>[2x]ERRRGLTDPEMAAVILKALPEAPLDGNNKMGYFVTPRWKRLTEYEALTVYAQPNADWIAGGLDWGDWTQKFHGGRPSWGNETTELRTVDWFKHRDPLRRWHAPYVKDKAEEWRYTDRFLQGYSADGQIRAMNPTWRDEFINRYWGAFLFNEYGLFNAHSQGAREALSDVTRVSLAFWGFDKIDIAQMIQLERGFLAKIVPGFDESTAVPKAEWTNGEVYKSARLAVEGLWQEVFDWNESAFSVHAVYDALFGQFVRREFFQRLAPRFGDNLTPFFINQAQTYFQIAKQGVQDLYYNCLGDDPEFSDYNRTVMRNWTGKWLEPTIAALRDFMGLFAKLPAGTTDKEEITASLYRVVDDWIEDYASRIDFKADRDQIVKAVLAGLK;>[2x]AANRAPTSVNAQEVHRWLQSFNWDFKNNRTKYATKYKMANETKEQFKLIAKEYARMEAVKDERQFGSLQVALTRLNAGVRVHPKWNETMKVVSNFLEVGEYNAIAATGMLWDSAQAAEQKNGYLAQVLDEIRHTHQCAYVNYYFAKNGQDPAGHNDARRTRTIGPLWKGMKRVFSDGFISGDAVECSLNLQLVGEACFTNPLIVAVTEWAAANGDEITPTVFLSIETDELRHMANGYQTVVSIAN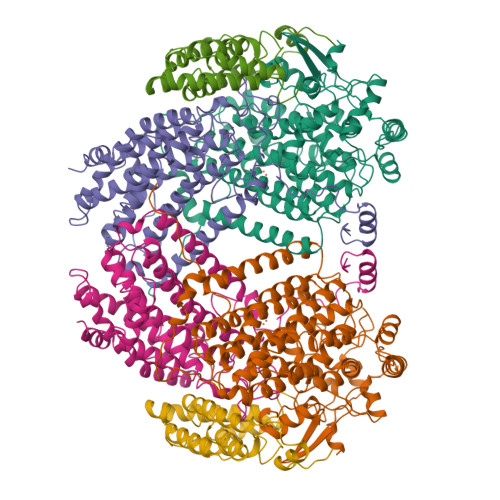DPASAKYLNTDLNNAFWTQQKYFTPVLGMLFEYGSKFKVEPWVKTWDRWVYEDWGGIWIGRLGKYGVESPRSLKDAKQDAYWAHHDLYLLAYALWPTGFFRLALPDQEEMEWFEANYPGWYDHYGKIYEEWRARGCEDPSSGFIPLMWFIENNHPIYIDRVSQVPFCPSLAKGASTLRVHEYNGEMHTFSDQWGERMWLAEPERYECQNIFEQYEGRELSEVIAELHGLRSDGKTLIAQPHVRGDKLWTLDDIKRLNCVFKNPVKAF;>LGIHSNDTRDAWVNKIAHVNTLEKAAEMLKQFRMDHTTPFRNSYELDNDYLWIEAKLEEKVAVLKARAFNEVDFRHKTAFGEDAKSVLDGTVAKMNAAKDKWEAEKIHIGFRQAYKPPIMPVNYFLDGERQLGTRLMELRNLNYYDTPLEELRKQRGVRVVH[2x]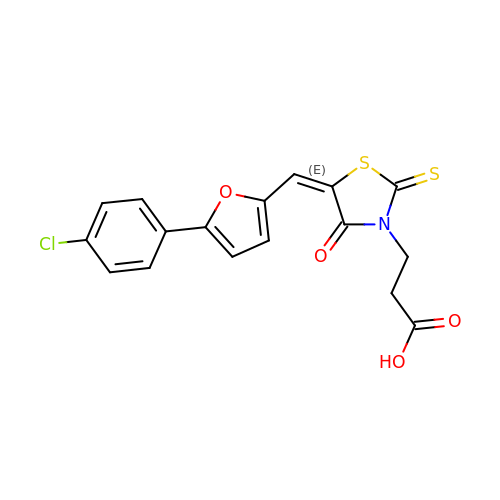(E)-3-(5((5-(4-CHLOROPHENYL)FURAN-2-YL)METHYLENE)-4-OXO-2-THIOXOTHIAZOLIDIN-3-YL)PROPANOIC ACID | C17 H12 Cl N O4 S2 | YZLFZFALAZYTCI-NTEUORMPSA-N>[2x]MVGLEDDTERERSPVVENGFSNGSRSSSSSAGVLSPSRKVTQGNDTLSYANILRARNKFADALALYEAMLEKDSKNVEAHIGKGICLQTQNKGNLAFDCFSEAIRLDPHNACALTHCGILHKEEGRLVEAAESYQKALMADASYKPAAECLAIVLTDLGTSLKLAGNTQEGIQKYYEALKIDPHYAPAYYNLGVVYSEMMQYDNALSCYEKAALERPMYAEAYCNMGVIYKNRGDLEMAITCYERCLAVSPNFEIAKNNMAIALTDLGTKVKLEGDVTQGVAYYKKALYYNWHYADAMYNLGVAYGEMLKFDMAIVFYELAFHFNPHCAEACNNLGVLYKDRDNLDKAVECYQMALSIKPNFAQSLNNLGVVYTVQGKMDAAASMIEKAILANPTYAEAFNNLGVLYRDA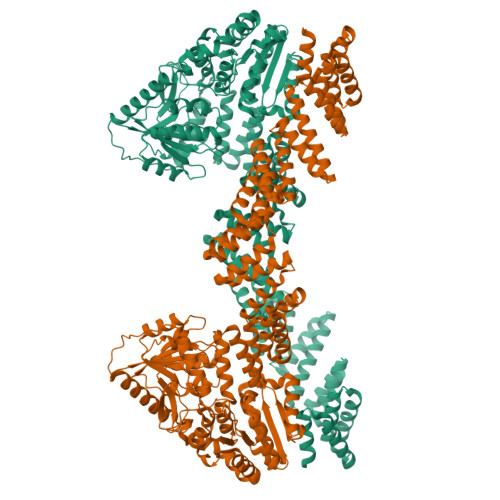GNITMAIDAYEECLKIDPDSRNAGQNRLLAMNYINEGLDDKLFEAHRDWGWRFTRLHPQYTSWDNLKDPERPITIGYISPDFFTHSVSYFIEAPLTHHDYTKYKVVVYSAVVKADAKTYRFRDKVLKKGGVWKDIYGIDEKKIASMVREDKIDILVELTGHTANNKLGTMACRPAPVQVTWIGYPNTTGLPTVDYRITDSLADPPDTKQKQVEELVRLPDCFLCYTPSPEAGPVCPTPALSNGFVTFGSFNNLAKITPKVLQVWARILCAVPNSRLVVKCKPFCCDSIRQRFLTTLEQLGLESKRVDLLPLILFNHDHMQAYSLMDISLDTFPYAGTTTTCESLYMGVPCVTMAGSVHAHNVGVSLLTKVGLGHLVAKNEDEYVQLSVDLASDVTALSKLRMSLRDLMAGSPVCNGPSFAVGLESAYRNMWKKYCKGEVPSLRRMEMLQKEVHDDPLISKDLGPSRVSVTGEATPSLKANGSAPVPSSLPTQSPQLSKRMDSTSGGSENLYFQGGSHHHHHHHHHHGGWSHPQFEK>[5x]GAMNEAVKTLDGWFCLHDFRSIDWAAWRELNPGNQELMLNELSHFLSDMEITKNIGEGEHTIYSILGQKADLVFFTLRDSLEALNEVENRFNKLAIADYLLPTYSYISVVELSNYLASHMAGGDDPYQNKGVRARLYPALPPKKHICFYPMSKKRDGADNWYMLPMEERQQLIRDHGLIGRSYAGKVQQIIGGSIGFDDYEWGVTLFSDDALEFKRIVTEMRFDEASARYAEFGSFFIGNLLLSEQLSKLFTI

Chlorite dismutase-like proteins are structurally closely related to functional chlorite dismutases which are heme b-dependent oxidoreductases capable of reducing chlorite to chloride with simultaneous production of dioxygen. Chlorite dismutase-like proteins are incapable of performing this reaction and their biological role is still under discussion. Recently, members of this large protein family were shown to be involved in heme biosynthesis in Gram-positive bacteria, and thus the protein was renamed HemQ in these organisms. In the present work the structural and heme binding properties of the chlorite dismutase-like protein from the Gram-positive pathogen Listeria monocytogenes (LmCld) were analyzed in order to evaluate its potential role as a regulatory heme sensing protein.

A crystal structure of apo-LmCld was solved and refined at a resolution of 2.0 Å. The overall structure of apo-LmCld subunit is composed of an N- and a C-terminal ferredoxin-like domain, as also observed in other Clds. In the crystal lattice apo-LmCld forms a homopentamer, compared to the hexameric assembly in solution. No electron density corresponding to heme was detected in the active site cavity of the C-terminal ferredoxin-like domain, despite the presence of a potential histidine residue as proximal ligand. In functional Clds a hydrogen bond between the proximal histidine and a neighboring glutamate stabilizes the position of the heme ligand. In contrast, an alanine replaces the glutamate in apo-LmCld. The distal site differs in having a glutamine residue at the position of the distal arginine which was shown to be of high importance for catalytic chlorite degrading activity. Moreover, similar to the Cld-like proteins from T. thermophilus and G. stearothermophilus, apo-LmCld contains a flexible stretch of amino acids between residues V105 and K141, as indicated by higher temperature factors and weaker electron density for these residues. This flexible stretch of residues aligns with the substrate channel forming α-helix of chlorite degrading chlorite dismutases and has a major impact on the access to the heme binding site, as shown by tunnel calculations in the respective proteins using CAVER. While in NdCld the access to the heme is very large, in apo-LmCld the access is significantly different and narrower, since the flexible stretch of amino acids is positioned in front of the putative heme binding site, as also reflected in diverse characteristics of the access channels.> GSHMASPNGQTKPLPALKLALEYIVPCMNKHGICVVDDFLGKETGQQIGDEVRALHDTGKFTDGQLVSQKSDSSKDIRGDKITWIEGKEPGCETIGLLMSSMDDLIRHCNGKLGSYKINGRTKAMVACYPGNGTGYVRHVDNPNGDGRCVTCIYYLNKDWDAKVSGGILRIFPEGKAQFADIEPKFDRLLFFWSDRRNPHEVQPAYATRYAITVWYFDADERARAKVKYLTGE;> ELDLETLAPYIPMDGEDFQL

The hypoxia‐inducible factor (HIF) prolyl‐hydroxylases (human PHD1‐3) catalyze prolyl hydroxylation in oxygen‐dependent degradation (ODD) domains of HIFα isoforms, modifications that signal for HIFα proteasomal degradation in an oxygen‐dependent manner. The PHDs and FIH are both Fe(II) and 2‐oxoglutarate (2OG)‐dependent oxygenases that couple hydroxylation with the conversion of 2OG to succinate and CO2. Crystal structures of PHD2.HIFα‐ODD complexes and kinetic studies have revealed the importance of a conformationally mobile loop (the β2–β3 loop) that links β2 and β3 of the catalytic domain of PHD2 and which is involved in HIFα‐ODD binding and selectivity; in the PHD2.substrate complexes, the β2–β3 loop folds to isolate the HIFα‐ODD substrate proline at the active site. Here, we report high‐resolution crystal structures of the truncated catalytic domain of PHD2 (residues 181–407) in complex with HIF2α‐CODD (residues 523–542), a manganese ion, and 2OG or its close isostere N‐oxalylglycine (NOG).

28 We added 3C with the aim of promoting crystallization of the PHD2181‐407.Mn.NOG.HIF2α‐CODD complex. The NOG and 2OG structures are very similar to each other (backbone RMSD: 0.078 Å) and, to a somewhat lesser extent in terms of details, with other PHD2.HIFα‐ODD structures. The previously reported PHD2 active site chemistry is also conserved in the PHD2181‐407.Mn.NOG/2OG.HIF2α‐CODD structures, 37 with a single manganese ion (substituting for iron) being coordinated by the side chains of His313, Asp315, and His374, as well as a well‐defined water molecule/hydroxide ion. 38 2OG and NOG bind the manganese ion in a bidentate manner via their C1 carboxylate and C2 carboxylate oxygens. The 2OG and NOG C5 carboxylates are positioned to interact with the guanidino group of Arg383. Although the overall PHD2181‐407.HIF2α‐CODD structures with NOG and 2OG are very similar (RMSD: 0.078 Å), there are some differences in the conformations of the β2–β3 loop involving PHD2 residues Gln243‐Asp246. In the 2OG.HIF2α‐CODD complex, the side chain amide NΗ2 group of PHD2 Gln243β2–β3 is positioned to form a hydrogen bond (2.74 Å) with the main chain carbonyl O atom of PHD2 Asp246. This hydrogen bond is, however, not observed in the NOG.HIF2α‐CODD complex, where Gln243β2–β3 is oriented away from the loop and adopts a more solvent‐exposed position. Although further work is required, given the 2OG and isostreric NOG structures have the same space group and similar crystal packing, the differences in the β2–β3 loop between them suggests that small differences at the active site region may influence the conformation of relatively distant structural elements within PHD2181‐407. 46 It is also of interest because it supports the previous proposal that inhibition by 2OG mimetics involves effects on structural dynamics in addition to simple blockade of 2OG binding in the active site.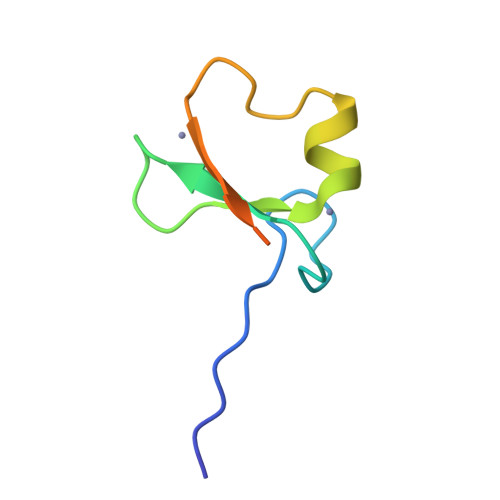>HEEEDVICDGCNGPVVGTRYKCSVCPDYDLCSVCEGKGLHRGHTKLAFPSPFGHLSEGFS[4x]> SMAKLSVSVEVPLPPEQAWEYASDLSRYHEWLSIHRAWRSKLPETLEKGTVIESIVEVKGMLNRVRWTLVHYKPPQALTLNGDGRGGVKVKLIGKIKP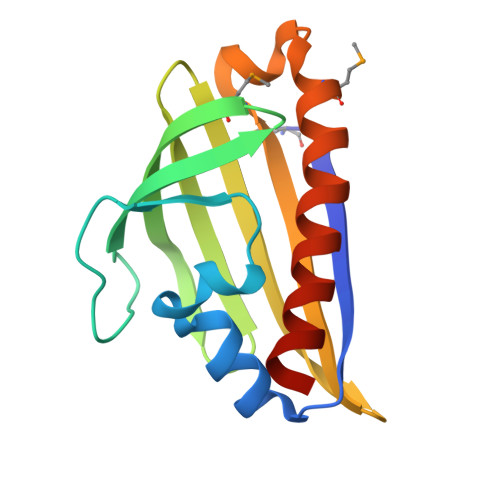TDNGATVGFDLHLGGPALFGPIGMVVAAALKSDIQESLNRFKQLYAPSAT> VDCSEYPKPACTSEYRPLCGSDNKTYGNKCNFCNAVVESNGTLTLSHF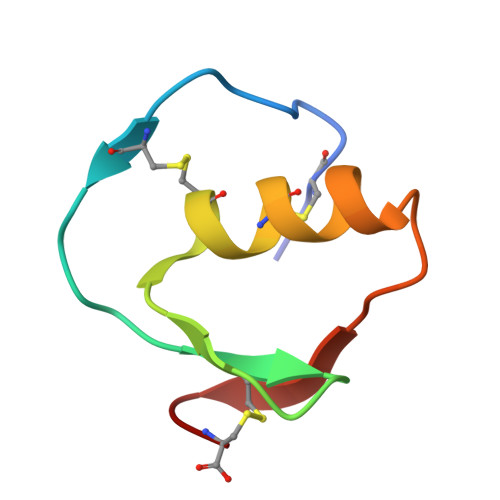GKC> SIPPEVKFNKPFVFLIIEQNT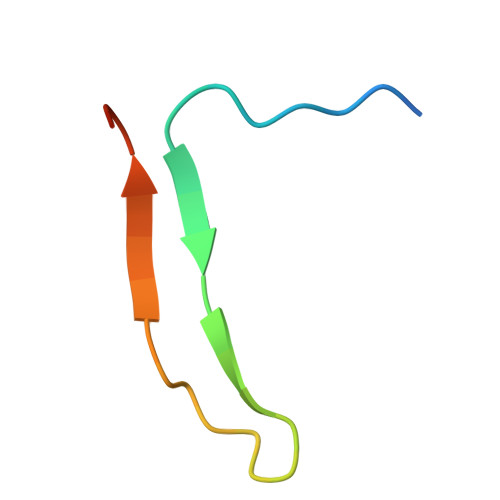KAPLFMGRVVNPTQK>MKSYEIALIGNPNVGKSTIFNALTGENVYIGNWPGVTVEKKEGEFEYNGEKFKVVDLPGVYSLTANSIDEIIARDYIINEKPDLVVNIVDATALERNLYLTLQLMEMGANLLLA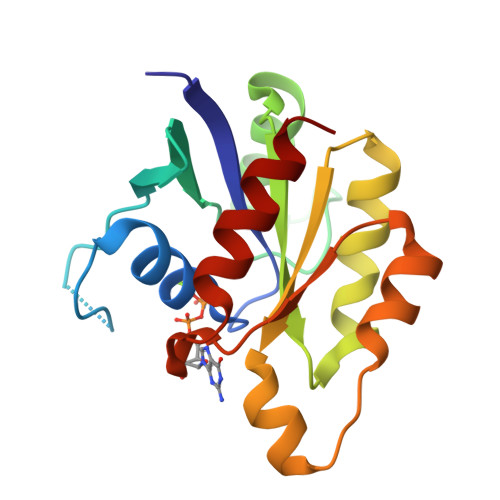LNKMDLAKSLGIEIDVDKLEKILGVKVVPLSAAKKMGIEELKKAISIAVKD[2x]> MSLKINQAIISVFIHETEDYNKIVNTIESFFSPLISNSKKNVTTAQGHYGNKIIILEYRFDRKSGEQFFKIILEKIETSELMLILTTIDSHIDGSKLYLRFDKQYLIAEHRLVLKEGDDVIKCIISFNTSLENIKEEIKKLVNSRIMHSKLEGHHHHHH

UPF0201 family proteins constitute one such uncharacterized, archaeal specific protein family. The UPF0201 family proteins occur as a single globular α/β domain with approximate dimensions of 55×35×35 Å3. The protomeric structure consists of a five-stranded, anti-parallel β-sheet, five α helices, which are located on one face of the β-sheet, and three loops connecting helices and strands. We have further documented that all members of this archaeal specific protein family share a common polypeptide chain fold, which is evolutionarily related to the RRM motif found in the ribosomal L5 proteins and many other RNA-binding proteins.

For 10077b and 10077c from S. solfataricus and S. solfataricus P2, respectively, full-length constructs bearing C-terminal His6 tags yielded crystals and structures. Our four UPF0201 structures represent subfamilies N149845 (10077a, b) and N130963 (10077c, d). The crystallographic asymmetric units contain one protomer in 10077c, two in 10077b and four protomers in both 10077a and 10077d. While 10077a, 10077b and 10077d all form one type of dimer (typeI), 10077c forms altogether different dimer via crystallographic symmetry (typeII). For type II dimer in 10077c, the interface surface area is larger and equal to 982 Å2. At the type II interface the turn connecting -strand β1 and helix α2 interacts with the turn that connects helix α4 and β5 (residues Gly115-Asp117). Majority of the interactions seen at the type II assembly interface are due to exchange of strands β2, β3, and the turn connecting them (residues Gly25-Asp50) between the two monomers. Moreover, this part of the structure in 10077c is about 5 residues longer compared to the other three. The interactions involve a large number of residues, which include Ser9, His13, Glu14, Thr15, Glu16, Asp17, His46, Asn49, Glu55, Asp116 and Gly117 of 10077c. Despite that the type II assembly involves large number of interactions and presumably more stable than the type I, such an assembly is seen only in one among the four structures reported here.> MDQKILSLAAEKTADKLQEFLQTLREGDLTNLLQNQAVKGKVAGALLRAIFKGSPCSEEAGTLRRRKIYTCCIQLVESGDLQKEIVSEIIGLLMLEAHHFPGPLLVELANEFISAVREGSLVNGKSLELLPIILTVLATKKENLAYGKGVLSGEECKKQLINTLCSGRWDQQYVIQLTSMFKDVPLTAEEVEFVVEKALSMFSKMNLQEIPPLVYQLLVLSSKGSRKSVLEGIIAFFSALDKQHNEEQSGDELLDVVTVPSGELRHVEGTIILHIVFAIKLDYELGRELVKHLKVGQQGDSNNNLSPFSIALLLSVTRIQRFQDQVLDLLKTSVVKSFKDLQLLQGSKFLQNLVPHRSYVSTMILEVVKNSVHSWDHVTQGLVELGFILMDSYGPKKVLDGKTIETSPSLSRMPNQHACKLGANILLETFKIHEMIRQEILEQVLNRVVTRASSPISHFLDLLSNIVMYAPLVLQNCSSKVTEAFDYLSFLPLQTVQRLLKAVQPLLKVSMSMRDCLILVLRKAMFANQLDARKSAVAGFLLLLKNFKVLGSLSSSQCSQSLSVSQVHVDVHSHYNSVANETFCLEIMDSLRRCLSQQADVRLMLYEGFYDVLRRNSQLANSVMQTLLSQLKQFYEPEPDLLPPLKLEACILTQGDQISLQEPLDYLLCCIQHCLAWYKNTVIPLQQGEEEEEEEEAFYEDLDDILESITNRMIKSELEDFELDKSADFSQSTSIGIKNNISAFLVMGVCEVLIEYNFSISSFSKNRFEDILSLFMCYKKLSDILNEKAGKAKTKMANKTSDSLLSMKFVSSLLTALFRDSIQSHQESLSVLRSSNEFMRYAVNVALQKVQQLKETGHVSGPDGQNPEKIFQNLCDLTRVLLWRYTSIPTSVEESGKKEKGKSISLLCLEGLQKIFSAVQQFYQPKIQQFLRALDVTDKEGEEREDADVSVTQRTAFQIRQFQRSLLNLLSSQEEDFNSKEALLLVTVLTSLSKLLEPSSPQFVQMLSWTSKICKENSREDALFCKSLMNLLFSLHVSYKSPVILLRDLSQDIHGHLGDIDQDVEVEKTNHFAIVNLRTAAPTVCLLVLSQAEKVLEEVDWLITKLKGQVSQETLSEEASSQATLPNQPVEKAIIMQLGTLLTFFHELVQTALPSGSCVDTLLKDLCKMYTTLTALVRYYLQVCQSSGGIPKNMEKLVKLSGSHLTPLCYSFISYVQNKSKSLNYTGEKKEKPAVVATAMARVLRETKPIPNLIFAIEQYEKFLIHLSKKSKV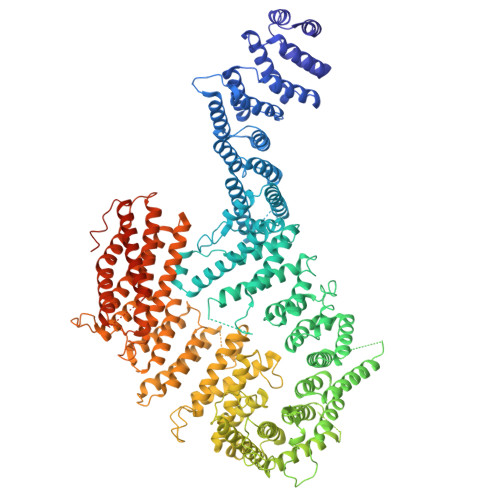SLMQHMKLSTSRDFKIKGNILDMVLREDGEDENEEGTASEHGGQNKEPAKKKRKK>HLIPPLNFSMVDNGIFRSGFPDSANFSFLQTLGLRSIIYLCPEPYPESNLQFLKSNGIRLFQFGIEGNKEPFVNIPDHKIRMALKVLLDEKNHPVLIHCKRGKHRTGCLVGCLRKLQKWCLTSIFDEYQRFAAAKA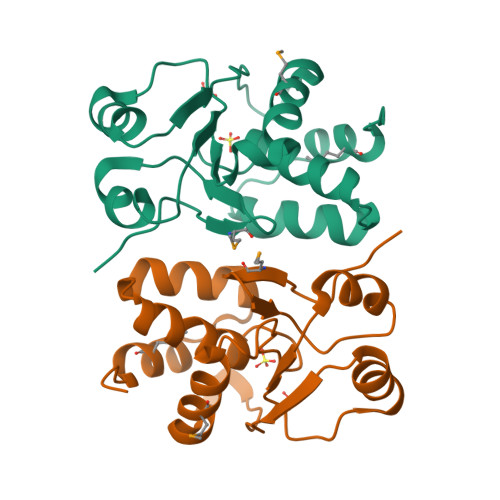RVSDQRFMEIFDVSS[2x]> MGTPALDTAQFTDAYKKANKRLLLFNYDGTLTPIVKVPSHAVPTERTRNAIAALCKDPKNVVYLISGRDGDFLEEHWGHLDRLGLSAEHGSFVKQPGEEDFINMTEALDMSWM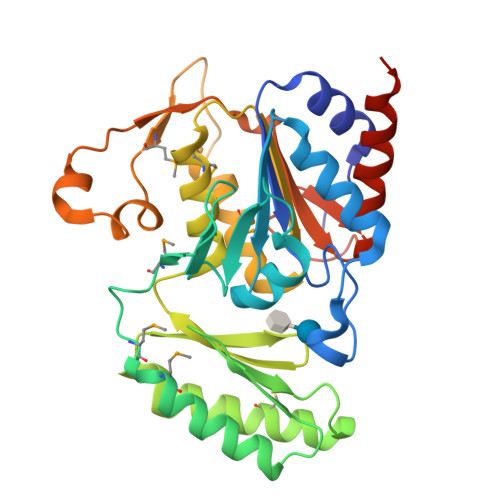SEVEEIFKYYTERTTGSTIEVKKASITWHYRNSDPDFGEFQCKQALDLLESSLAPRRPIEVLVGKKNLEVRPLAVNKGEIVRRLMYENPDVDLIFCAGDDKTDEDMFRALRTIFPPGGVVDNNPVVMKPPVAVTSALEPEEVAELPDVELTIRSKGVFATTVGPPAKRTLAGWHVTCPEEVVEAFESLLEEIQVVLEHHHHHH> MEEIQGYDVEFDPPLESKYECPICLMALREAVQTPC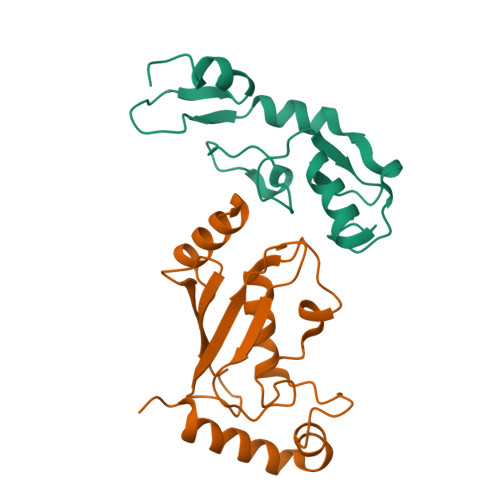GHRFCKACIIKSIRDAGHKCPVDNEILLENQLFPDNFAKREILSLMVKCPNEGCLHKMELRHLEDHQAHCEFALLEHHHHHH;> GSHMAGLPRRIIKETQRLLAEPVPGIKAEPDESNARYFHVVIAGPQDSPFEGGTFKLELFLPEEYPMAAPKVRFMTKIYHPNVDKLGRICLDILKDKWSPALQIRTVLLSIQALLSAPNPDDPLANDVAEQWKTNEAQAIETARAWTRLYAMNNI> XVALDPIDXSIV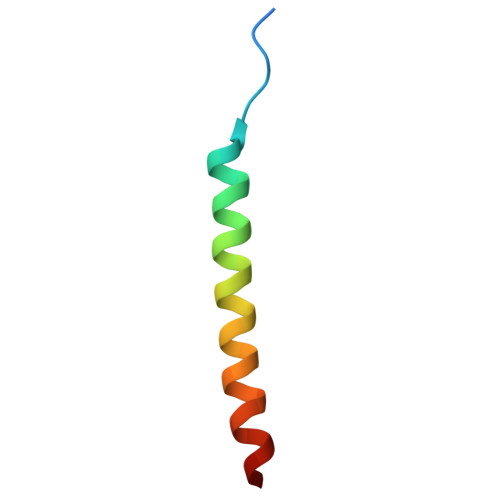LNKIKSQLEESKEWIRRSNKILDSIX>HHHHHHSSGLVPRGSHMSVKKAGVLGATGSVGQRFILLLSKHPEFEIHALGASSRSAGKKYKDAASWKQTETLPETEQDIVVQECKPEGNFLECDVVFSGLDADVAGDIEKSFVEAGLAVVSNAKNYRREKDVPLVVPIVNPEHIDVVENKVKQAVSKGGKKPGFIICISNCSTAGLVAPLKPLVEKFGPIDALTTTTLQAISGAGFSPGVSGMDILDNIVPYISGEEDKLEWETKKILGGVNAEGTEFVPIPESEMKVSAQCNRVPVIDGHTECISLRFANRPAPSVEDVKQCLREYECAASKLGCHSAPKQTIHVLDQPDRPQPRLDRDRDSGYGVSVGRIREDSLLDFKMVVLSHNTIIGAAGAGILIAEILKAKNII[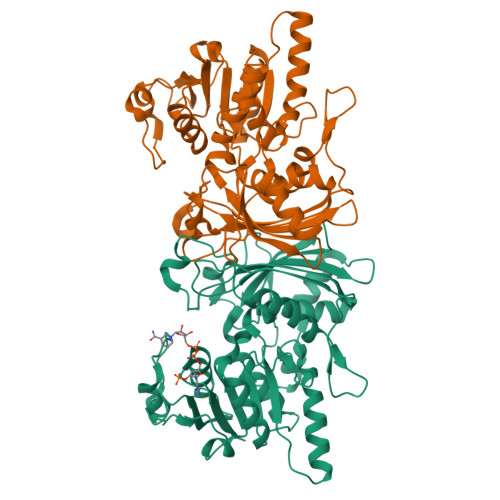2x]> STSRGMITDRSGRPLAVSVPVGGGESRRYYPSGEVTAHLIGFTNVDSQGIEGVEKSFDKWLTGQGGGAAHNLALSIDERLQALVYRELNNAVAFNKAESGSAVLVDVNTGEVLAMANSPSYNPNNLSGTPKEAMRNRTITDVFEPGSTVKPMVVMTALQRGVVRENSVLNTIPYRINGHEIKDVARYSELTLTGVLQKSSNVGVSKLALAMPSSALVDTYSRFGLGKATNLGLVGERSGLYPQKQRWSDIERATFSFGYGLMVTPLQLARVYATIGSYGIYRPLSITKVDPPVPGERVFPESIVRTVVHMMESVALPGGGGVKAAIKGYRIAIKTGTAKKVGPDGRYINKYIAYTAGVAPASQPRFALVVVINDPQAGKYYGGAVSAPVFGAIMGGVLRTMNIEPDALTT

Subclass B3 PBP (known as PBP3 in Escherichia coli and encoded by the ftsI gene) is active during cell division and localizes to a multiprotein complex termed the divisome, where it functions in PG synthesis in concert with the division-specific glycosyltransferase FtsW. PBP3 consists of three major domains: the N-terminal transmembrane helix anchors the protein in the cell membrane, while the C-terminal transpeptidase domain (TPd) is the catalytic module of PBP3 and mediates cross-linking of PG chains by ω-peptide linkages between d-Ala and meso-diaminopimelic acid (m-DAP) residues on opposing peptide chains. The catalytic serine acting as a nucleophile in the transpeptidation mechanism is also able to react with β-lactam antibiotics because of their structural similarity with the d-Ala-d-Ala motif; the resulting covalent intermediate, however, has a very long half-life (with turn-over constant k3 ~ 10−4 M−1s−1 or less), effectively leading to irreversible inactivation. AiCuris previously reported on the development of a novel monobactam (AIC499), which shows remarkable inhibitory activity against PBPs of Gram-negative bacteria, and good antibacterial activity, even against clinical isolates harboring several β-lactamase classes.

The EcPBP3ΔTM and EcTPd* proteins were crystallized after pre-incubation with the experimental β-lactam AIC499. In the case of the truncated version, the presence of the compound left the space group (P 62 2 2) and packing unchanged. It did, however, impart a notable improvement in useable resolution, along with slight changes in lattice constants. Since there were only negligible differences between the two models (RMS distance: 0.37 Å for 336 equivalent Cα positions), we will focus on the binding of AIC499 to EcTPd* because (i) electron density was clearly more informative in this structure, and (ii) despite differences in crystallization conditions, the complex has been crystallized in the same space group as the apo form, minimizing spurious differences caused by non-conserved lattice contacts. As expected for a β-lactam antibiotic, AIC499 is found as a covalent acyl-enzyme intermediate, with the carbonyl group of the hydrolyzed lactam forming an ester with the side chain oxygen of the catalytic S307. The compound adopts a U-shaped overall conformation, and its presence correlates with several conformational changes in the protein environment, mostly regarding the β2b-β2c-β2d, β3-β4, and β5-α11 regions, which contribute to the upper lobe, the bottom, and the lower lobe, respectively, of the binding cleft. The largest differences between apo and complex structures can be observed in the β5-α11 region, in particular residues K539-A544. Being poorly ordered and not completely resolved in the native protein, this segment is well-structured when AIC499 is bound in the active site.>[2x]MAHHHHHHSSGLEVLFQGPADTLQSLAILGATGSIGDSTLAIIRQHPNRYRIHALTGFSRVDKLLALAMEFHPVKICTSPDNYAQLSQKVTDAGLDTIILSGDEGLIEIASDEAVDTVVAAIVGAAGLSSTLAAAGAGKRILLANKESLVMAGDLVIKTAKKHG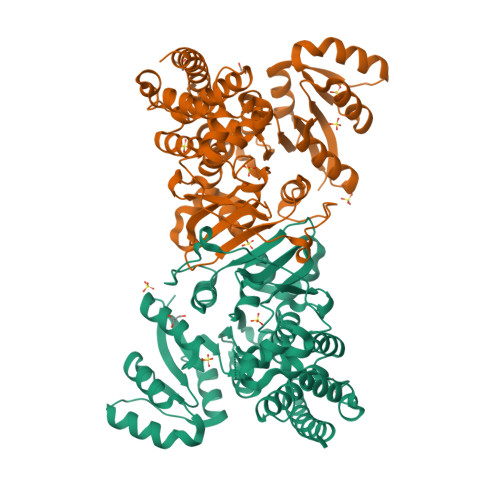ATILPIDSEHNAIYQCLPAAIQADNTAIHHTSYGIKKLWLTASGGSFLDKSIKQMQNASVKEAVNHPNWSMGQKISIDSATMMNKGLELIEACHLFDLKEHQIQVVIHPNSVVHSLVEYVDGSFLAQLGTPDMKTPIAHALAYPERIKSGVMPLDLYQLGSLKFLAPDLDKFACLKLARYAARLGTGACIALNTANEIAVEAFLAEKICLTDIAVIVKACLDDKTIAQDYSQDFGDEVLGLERILTMDKKVRKIATAKIKLLKQGDVL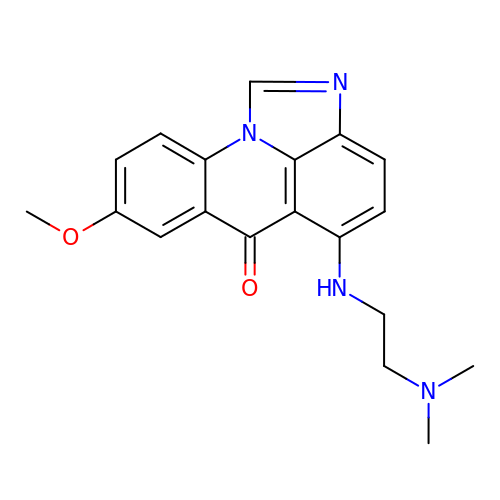5-{[2-(dimethylamino)ethyl]amino}-8-methoxy-6H-imidazo[4,5,1-de]acridin-6-one | C19 H20 N4 O2 | NJTQMNXHSDDMHX-UHFFFAOYSA-N> MATDVAQGPNGRALAESMNPDLLSAIQQHISIERYASVT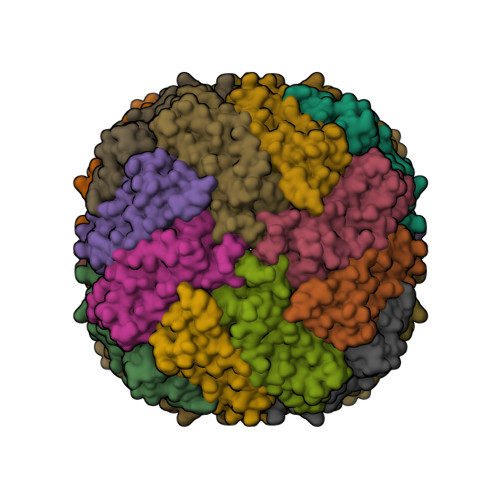YLAMSIWCAERELAGFYQFFDGEAKAEQSHAVHFTQYLIARSQSNDLQTLDAPRQNWDSLASLMATAFQMEADTTSSIQSVYALAERNSDTRTTVFLDPLIEAQIQSEDQFAYLLGRVKFANGDPTALLVIDNELRAGQTQRG Using a pair of evolutionarily related DNA-binding proteins, each with a different DNA preference (ParB [Partitioning Protein B] and Noc [Nucleoid Occlusion Factor], which both play roles in bacterial chromosome maintenance), we show that specificity is encoded by a set of four residues at the protein-DNA interface. Like ParB, Noc has a three-domain architecture: an N-terminal domain for protein-protein interactions and for targeting Noc to the cell membrane, a central DNA-binding domain (DBD), and a C-terminal dimerization domain (Wu and Errington, 2004; Wu et al., 2009). The NBS site differs from the parS site by only 2 bases (positions 1 and 6), but Noc and ParB recognize and bind them with exquisite specificity. We show that specificity to parS or NBS is encoded by a small set of four residues at the protein-DNA interface and that mutations in these residues are enough to reprogram DNA-binding specificity.

To understand the biophysical mechanism underlying the specificity to NBS, we solved the co-crystal structure of B. subtilis Noc (DBD) with a 22-bp NBS DNA duplex. The diffraction of the Noc (DBD)-NBS crystal was anisotropic. Hence, despite the 2.23-Å resolution limit, because of low completeness in the higher resolution shells resulting from the anisotropic cutoff, the resultant electron density has the appearance of lower resolution maps, approximately a 3-Å resolution (STAR Methods). In contrast to ParB, Noc recognizes a DNA-binding sequence called NBS (Noc Binding Site) (Pang et al., 2017; Wu et al., 2009). The role of Noc is also different from ParB; Noc functions to prevent the cell division machinery from assembling in the vicinity of the nucleoid, which might be otherwise guillotined, thereby damaging the DNA (Wu and Errington, 2004; Wu et al., 2009: Figure 1B). By superimposing the structures of ParB (DBD)-parS and Noc (DBD)-NBS complexes, we observed several changes in both the protein and the DNA sites that enabled specific interactions. However, a corresponding base in NBS (adenine 1) positions itself closer to enable hydrogen bonding with this Q173 residue; this is possibly due to conformational changes in the NBS site that narrows the minor groove width at the adenine 1:thymine −1 position (from ~7.7 to ~3.7 Å). However, the equivalent residue R186 in Noc readily forms hydrogen bonds with guanine −6. We also observed DNA unwinding that increased both the minor and the major groove widths at the cytosine 6:guanine −6 position of NBS (from ~7.1 to ~8.1 Å and from ~10.5 to ~11.8 Å, respectively), possibly to move guanine −6 outward to accommodate a longer side chain of arginine. Our Noc (DBD)-NBS structure also shows the side chains of K164 and K169 make hydrogen bonds with the phosphate groups of guanine −5 and thymine 2 of NBS rather than contacting any bases specifically.

>MTETASVALIENLQREELSSIEEAHAYARLLELHDLTQEALAQRLGKGQSTIANKLRLLKLPQPVQEAIMEKKITERHARALIPLKQPELQVTLLTEIIEKSLNVKQTEDRVVKMLEQGQRKPKPRRKAFSRDKLAAALEHHHHHH[2x]>MRCIGISNRDFVEGVSGGSWVDIVLEHGSCVTTMAKNKPTLDFELIKTEAKQPATLRKYCIEAKLTNTTTDSRCPTQGEPSLNEEQDKRFVCKHSMVDRGWGNGCGLFGKGGIVTCAMFTCKKNMKGKVVQPENLEYTIVITPHSGEEHAVGNDTGKHGKEIKITPQSSITEAELTGYGTVTMECSPRTGLDFNEMVLLQMENKAWLVHRQWFLDLPLPWLPGADTQGSNWIQKETLVTFKNPHAKKQDVVVLGSQEGAMHTALTGATEIQMSSGNLLFTGHLKCRLRMDKLQLKGMSYSMCTGKFKVVKEIAETQHGTIVIRVQYEGDGSPCKIPFEIMDLEKRHVLGRLITVNPIVTEKDSPVNIEAEPPFGDSYIIIGVEPGQLKLNWFKKGSSIGQMIETTMRGAKRMAILGDTAWDFGSLGGVFTSIGKALHQVFGAIYGAAFSGVSWIMKILIGVIITWIGMNSRSTSLSVSLVLVGVVTLYLGVMVQA[72x];>FHLTTRNGEPHMIVSRQEKGKSLLFKTEDGVNMCTLMAMDLGELCEDTITYKCPFLKQNEPEDIDCWCNSTSTWVTYGTCTTTGEHRREKRSVALVPHVGMGLETRTETWMSSEGAWKHAQRIETWILRHPGFTIMAAILAYTIGTTHFQRALIFILLTAVAPSMT[72x]

Flavivirus envelope (E) and precursor M (prM) proteins, when ectopically expressed, assemble into empty, virus-like particles (VLPs). Cleavage of prM to M and loss of the pr fragment converts the VLPs from immature to mature particles, mimicking a similar maturation of authentic virions. The icosahedrally symmetric, immature particles contain 180 envelope (E) subunits associated with the same number of membrane-protein precursor (prM) subunits and internal, core (C) protein subunits. Both E and prM are glycoproteins with C-terminal, transmembrane anchors. We describe here the cryo-EM structure of immature, small VLPs (smVLPs) from dengue virus type 2 and show that they have octahedral rather than icosahedral symmetry.

We obtained a 3D reconstruction of an immature DENV2 smVLP at 6.5 Å resolution. We show here that immature smVLPs of dengue virus type 2 (DENV2), and by extension those of other flaviviruses, are octahedrally symmetric particles, with prM-E asymmetrically clustered as on immature virions. The octahedral asymmetric unit is one asymmetric cluster of three prM-E heterodimers, and thus, there are 72 prM-E heterodimers in total. Early work suggested that the smVLPs of TBEV were 60-subunit, icosahedral particles. But because icosahedral symmetry for a 60-subunit surface requires symmetric threefold clusters, it is incompatible with the asymmetric threefold clusters now known (from work that came several years later) to be present on immature virions and presumably on the smVLPs. The sharper curvature of the particle displaced the transmembrane segments from their positions, relative to their ectodomains, in the 180-subunit, immature flavivirions for which subnanometer structures are known (Data sets S4 and S5). The ovoid mature smVLPs appear to have various local compromises, varying across a particle and between particles; those local packings might include instances of the one that would characterize the fully octahedral alternative.> MPLTGLEIYKQLPKKNCGECGTPTCLAFAMNLASGKASLDSCPYVSDAAREALDAAAAPPIAKVVLGAGPTAVEMGDETELFRHDKRFYHETAIAIQVSDNLSSEELKAKVEAINGLNFDRVGQHYTIQAIAIRHDADDPAAFKAAVASVAAATQLNLVLMADDPDVLKEALAGVADRKPLLYAATGANYEAMTALAKENNCPLAVYGNGLEELAELVDKIVALGHKQLVLDPGARETSRAIADFTQIRRLAIKKRFRSFGYPIIALTTAANPLDEVLQAVNYVTKYASLVVLRTDAKEHLLPLLSWRQNLYTDPQVPIRVEEKLNEIGAVNENSPVYVTTNFSLTYYSVEGEIESTKIPSYLLSVDTDGLSVLTAYADGKFEAEKIAAVMKKVDLDNKVKRHRIIIPGAVAVLKGKLEDL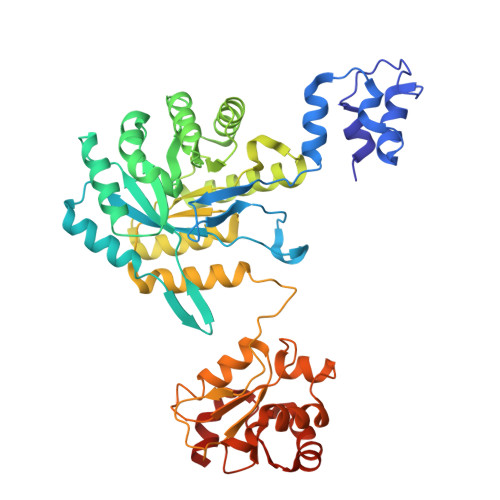TGWEVIVGPREASGIVAFARANLAS>[2x]MNNSKIISKVLLSLSLFTVGASAFVIQDELMQKKHAKAEVSAEEIKKHEEKWNKYYGVNAFNLPKELFSKVDEKDRQKYPYNTIGNVFVKGQTSATGVLIGKNTVLTNRHIAKFANGDPSKVSFRPSINTDDNGNTETPYGEYEVKEILQEPFGAGVDLALIRLKPDQNGVSLGDKISPAKIGTSNDLKDGDKLELIGYPFAHKVNQMHRSEIELTTLSRGLRYYGFTVPGNSG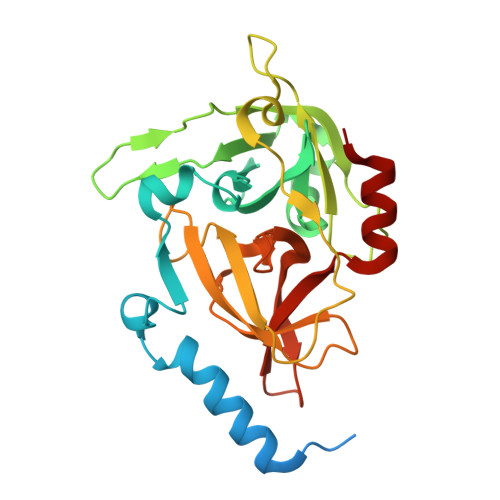SGIFNSNGELVGIHSSKVSHLDREHQINYGVGIGNYVKRIINEKNE> MFIKPGRCPKPAVQEDFDAARYLGVWYDIQRLPNKFQKGECATATYSLSPGVGFSVFNRERLANGTIKSVIGSAIAEDPCEPAKLQFFHENAAPVPYWVLSTDYDNYALVYSCINEGASHAAYASIVSRQPTLPEETIKKLQGTMSSFGVGVDTLLTTNQDAAYCSAMNQKLAAALEHHHHHH

Sandercyanin (SFP) is a BV-binding lipocalin protein found in the skin mucus of the Canadian walleye, Stizostedion vitreum (formerly Sander vitreus). BV associates non-covalently to each SFP monomer in a ZZZssa conformation and is stabilized by aromatic stacking, hydrophobic interactions, and water-mediated H-bonding inside the lipocalin-like beta-barrel fold of SFP. The binding of BV induces tetramerization of SFP via interaction between amino acid residues from adjacent monomeric subunits. Using a combination of designed site-directed mutations, X-ray crystallography, UV/VIS, and resonance Raman spectroscopy, we have identified multiple conformations of BV that are stabilized in the binding pocket of SFP.

Two mutations – L135E (from interface 1) and V71E (from interface 2) stayed monomers on binding to BV as identified by size-exclusion chromatography profiles. The absorbance spectra of BV-bound V71E and L135E show maxima at 380 nm and an attenuated red-shifted broad peak at the far-red wavelengths (∼680–700 nm) compared to the wild-type protein, where the red-absorbance is at 630 nm. The V71E and L135E mutations showed an order of magnitude reduction, with fluorescence quantum yields of 0.003 and 0.0025, respectively (for excitation at 630 nm). The overall fold of the monomeric variant proteins is very similar to the wild-type protein, with BV bound at the center of the barrel. In the BV-binding pocket, both monomeric variants revealed a rotated D-ring pyrrole of BV around the C14–C15 single bond. Measured torsion angles were 122° and 125° (counter-clockwise) for V71E and L135E, respectively. The conformation of BV is ZZZsss in the variants compared to ZZZssa in wild-type SFP. However, the atoms of the D-ring of the L135E have larger B-factors suggesting that even in the crystal structure, this ring is more flexible. However, in the monomeric forms, the orientation of the D-ring of BV is stabilized by interactions with the A-ring of BV (the D-ring moves closer to the A-ring of BV) and stacking interactions with the Y142 side chain (which rotates to stack with the D-ring). The lower resolution structure of L135E does not allow modeling of structured waters replacing the rotated residues; however, empty space possibly suggests randomly-oriented or the presence of low occupancy water molecules.Here, we present the crystal structure of C. acetobutylicum thiolase (CaTHL), a type II biosynthetic thiolase that catalyses the first step of n-butanol biosynthesis and condenses two acetyl-CoAs to acetoacetyl-CoA. We reveal that CaTHL, unlike other type II biosynthetic thiolases from aerobic bacteria, is regulated via modulation of a redox-switch, indicating that n-butanol production and the relevant metabolic fluxes in Clostridium are tightly regulated by thiolase. CaTHL consists of three domains: an N-terminal α/β domain (N-domain, residues 1–119 and 249–269), a loop domain (L-domain, residues 120–248), and a C-terminal α/β domain (C-domain, residues 270–392). The N- and C-domains form a typical five-layered fold (α–β–α–β–α) observed in other thiolase superfamily of proteins including peroxisomal degradative thiolase from Saccharomyces cerevisiae, β-ketoacyl synthase II from E. coli, and the biosynthetic thiolase from Zoogloea ramigera (ZrTHL)14151617181920.

On the basis of the finding that the instability of RDR confers the redox-switch regulatory mechanism to CaTHL, a CaTHL mutant CaTHLV77Q/N153Y/A286K was generated by introducing residues that might be able to form hydrogen bonds with their neighbours and subsequently increase the stability of the CaTHL RDR. Unlike the wild-type CaTHL, the activity of the H2O2-treated CaTHLV77Q/N153Y/A286K mutant could not be recovered by the addition of a reducing agent as similarly found for EcTHL and ZrTHL. To confirm the reason for this, the crystal structure of the CaTHLV77Q/N153Y/A286K mutant was determined at 2.3 Å resolution; it was structurally confirmed that there were the change of regulatory mechanism and the stability of RDR in the CaTHLV77Q/N153Y/A286K mutant. As expected, a disulfide bond formation was not observed between the catalytic cysteine residues in the CaTHLV77Q/N153Y/A286K mutant and the RDR was found to be tightly ordered, forming a sheet–turn–helix conformation even without the addition of a reducing agent. More interestingly, the mutated residues, V77Q, N153Y and A286K, were positioned to form hydrogen bonds with each other. These hydrogen bonds seem to contribute to the well-ordered conformation of the RDR in the CaTHLV77Q/N153Y/A286K mutant. When the thlCaV77Q/N153Y/A286K gene was overexpressed in the thlA-knockdown mutant under the control of its native promoter, n-butanol concentration (7.4 g l−1) was higher than that (4.5 g l−1) obtained with the thlA-knockdown mutant complemented with the thlCa.

>MKEVVIASAVRTAIGSYGKSLKDVPAVDLGATAIKEAVKKAGIKPEDVNEVILGNVLQAGLGQNPARQASFKAGLPQEIPAMTINKVCGSGLRTVSLAAQIIKAGDADVIIAGGMENMSRAPYLANNARWGYRMGNAKFVDEMITDGLWDAFYDYHMGITAENIAERWNISREEQDEFALASQKKAEEAIKSGQFKDEIVPVVIKGRKGETVVDTDEHPRFGSTIEGLAKLKPAFKKDGTVTAGNASGLNDCAAVLVIMSAEKAKELGVKPLAKIVSYGSAGVDPKIMGYGPFYATKAAIEKAGWTVDELDLIESNEAFAAQSLAVAKDLKFDMNKVNVNGGAIALGHPIGASGARILVTLVHAMQKRDAKKGLATLCIGGGQGTAILLEKCLEHHHHHH[2x]>[8x]ASMLPQVKALYPYTAANDEELSFKVGDIITILEKDEGWWKGELN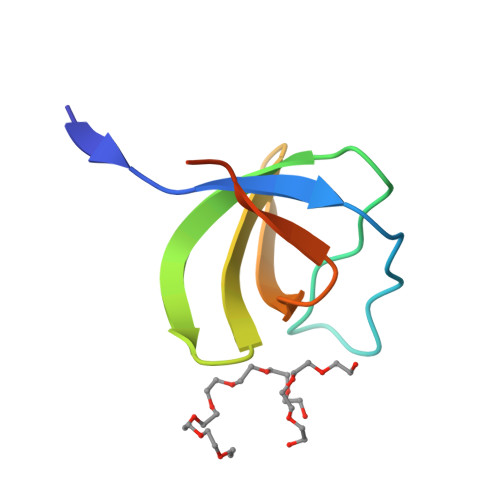GQEGWIPNNYVKEILEHHHHHH>[2x]GSMHLTARGLTLDLSRPQVMGILNVTPDSFSDGGCHNNLDQALQHAQRMLSAGATLIDIGGESTRPGAAEVSEQEELDRVVPVVEALAQRFDVWLSVDTSKAAVITESAHAGAHLINDIRSLQEPGALEAAAKTGLPVCLMHMQGQPKNMQHSPYYDDLMTDINRFFQHHIERCVAAGIAKNKLLLDPGFGFGKNLAHNYQLLAHLSELHHFELPLLVGMSRKSMVGQLLNVPPQQRVIGS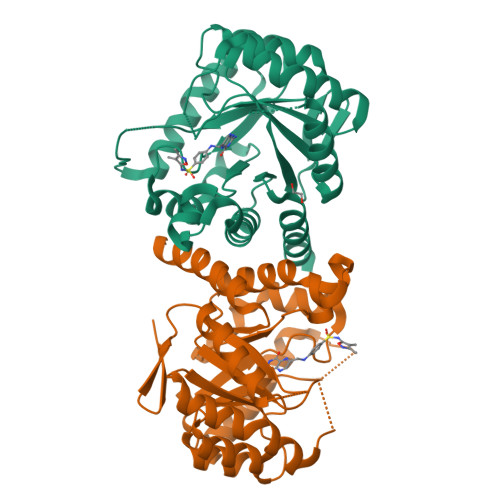VACAVIAAMQGAQIIRVHDVKETVEAMCIVEATRSAKG> AMSLNIITVTLNME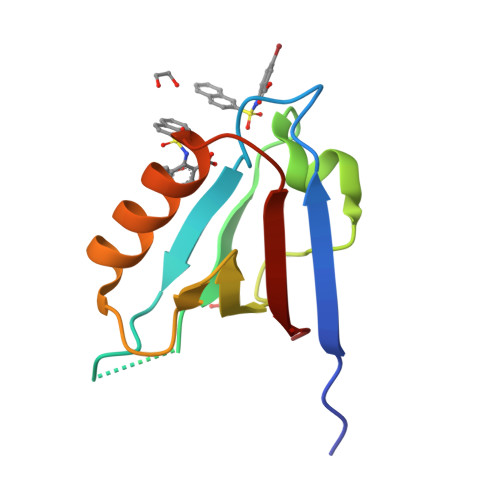KYNFLGISIVGQSNERGDGGIYIGSIMKGGAVAADGRIEPGDMLLQVNEINFENMSNDDAVRVLREIVHKPGPITLTVAKS(2R)-2-[(E)-[2-methyl-3-oxidanyl-5-(phosphonooxymethyl)pyridin-4-yl]methylideneamino]-3-sulfanyl-propanoic 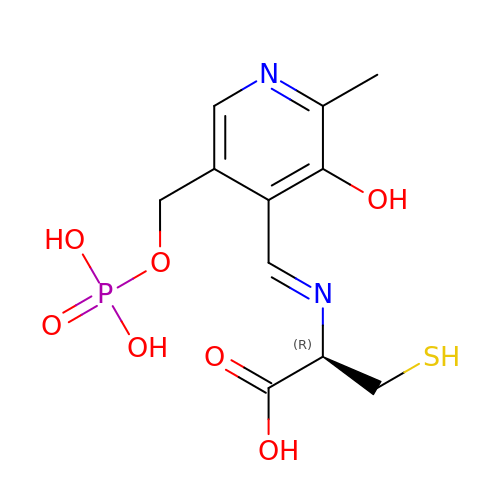acid | C11 H15 N2 O7 P S | NUTWYOJHALJXFM-BIMOUXMDSA-N>QKRAIYPGTFDPITNGHIDIVTRATQMFDHVILAIAASPSKKPMFTLEERVALAQQATAHLGNVEVVGFSDLMANFARNQHATVLIRGLRAVADFEYEMQLAHMNRHLMPELESVFLMPSKEWSFISSSLVK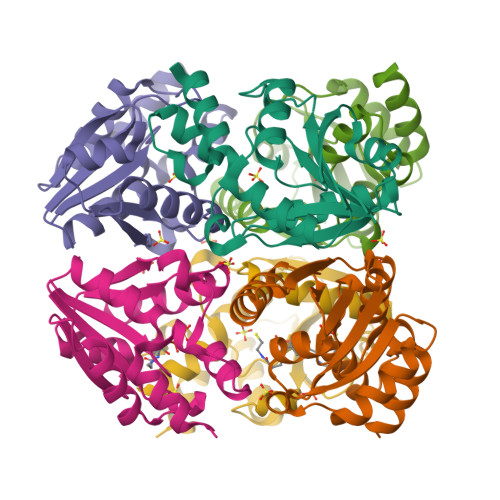EVARHQGDVTHFLPENVHQALMAKLA[2x]> HHHHHMPVFHTRTIESILEPVAQQISHLVIMHEEGEVDGKAIPDLTAPVAAVQAAVSNLVRVGKETVQTTEDQILKRDMPPAFIKVENACTKLVQAAQMLQSDPYSVPARDYLIDGSRGILSGTSDLLLTFDEAEVRKIIRVCKGILEYLTVAEVVETMEDLVTYTKNLGPGMTKMAKMIDERQQELTHQEHRVMLVNSMNTVKELLPVLISAMKIFVTTKNSKNQGIEEALKNRNFTVEKMSAEINEIIRVLQLTS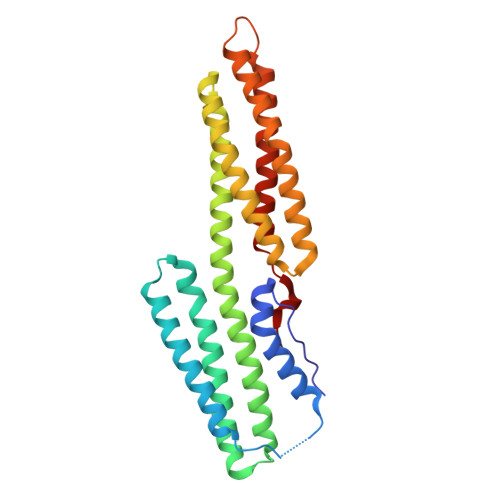WDEDAW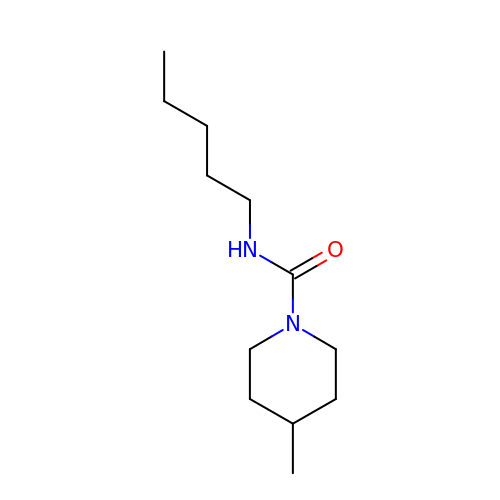4-methyl-~{N}-pentyl-piperidine-1-carboxamide | C12 H24 N2 O | ZVWQTTCMILVTNG-UHFFFAOYSA-N3-(3-fluorophenyl)-N-{2-[2-(1H-imidazol-1-yl)pyrimidin-4-yl]ethyl}propan-1-amine 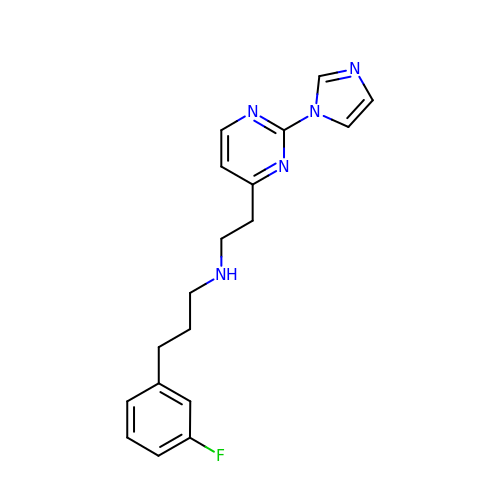| C18 H20 F N5 | GTABKUMYLUXCIH-UHFFFAOYSA-N Human calcium-sensing receptor (CaSR) is a G-protein-coupled receptor (GPCR) that senses small fluctuations of extracellular levels of Ca2+ ions in the blood. It maintains Ca2+ homeostasis by the modulation of parathyroid hormone (PTH) secretion from parathyroid cells and the regulation of Ca2+ reabsorption by the kidney. Like most class C GPCRs, CaSR functions as a disulphide-linked homodimer. In this study, we have determined the cryo-EM structures of CaSR in the fully inactive and agonist+PAM bound states.

To obtain the structure of the receptor in the agonist+PAM bound state, we collected a dataset of detergent solubilized full-length CaSR in the presence of PAM cinacalcet, 10 mM calcium and the compound TNCA. We have observed two active conformations with overall resolutions of 2.99 Å and 3.43 Å. The agonist+PAM bound structure of CaSR displays a substantial compaction compared to the inactive structure, including the reduction of length, height, and width. Moreover, their width changed most obviously because there are four interfaces with interaction between the two protomers at each of LB1 domain, LB2 domain, CRD, and 7TM domains, both VFT modules adopt closed–closed conformation, and the TNCA and Ca2+ ion composite is bound at the interdomain cleft between LB1 domain and LB2 domain. The cryo-EM map of active state presents a distinct density at the ligand-binding cleft of each protomer, which enabled us to unambiguously model TNCA. Two sites were previously reported, while a new Ca2+-binding site was found at the interdomain cleft of the VFT module that is close to the hinge loop and abuts the TNCA binding site, and interacts with both LB1 and LB2 domains to facilitate ECD closure. The bound Ca2+ ion is primarily coordinated with side chains of D190 and E297, carbonyl oxygen atoms of P188 backbone, and hydroxyl groups of S170 and Y489. Our CaSRagonist+PAM structure shows that TNCA and a newly identified Ca2+ ion bind at the interdomain cleft of the VFT module, and they both interact with both LB1 and LB2 domains to facilitate ECD closure, therefore forming the closed state of the ligand-binding domain required for CaSR activation. The agonist+PAM bound structure shows a TM6–TM6 interface, contacting at the apex of TM6 helices, which is a hallmark of GPCR activation (Koehl et al., 2019). In the agonist+PAM bound state, the loop of ECL2 is pulled up by the interaction among E759, W590, and K601, leading to the movement of ECL2, which would raise the reorientation of TM5 and TM6 domains during the activation of CaSR.

>YGPDQRAQKKGDIILGGLFPIHFGVAAKDQDLKSRPESVECIRYNFRGFRWLQAMIFAIEEINSSPALLPNLTLGYRIFDTCNTVSKALEATLSFVAQNKIDSLNLDEFCNCSEHIPSTIAVVGATGSGVSTAVANLLGLFYIPQVSYASSSRLLSNKNQFKSFLRTIPNDEHQATAMADIIEYFRWNWVGTIAADDDYGRPGIEKFREEAEERDICIDFSELISQYSDEEEIQHVVEVIQNSTAKVIVVFSSGPDLEPLIKEIVRRNITGKIWLASEAWASSSLIAMPQYFHVVGGTIGFALKAGQIPGFREFLKKVHPRKSVHNGFAKEFWEETFNCHLQEGAKGPLPVDTFLRGHEESGDRFSNSSTAFRPLCTGDENISSVETPYIDYTHLRISYNVYLAVYSIAHALQDIYTCLPGRGLFTNGSCADIKKVEAWQVLKHLRHLNFTNNMGEQVTFDECGDLVGNYSIINWHLSPEDGSIVFKEVGYYNVYAKKGERLFINEEKILWSGFSREVPFSNCSRDCLAGTRKGIIEGEPTCCFECVECPDGEYSDETDASACNKCPDDFWSNENHTSCIAKEIEFLSWTEPFGIALTLFAVLGIFLTAFVLGVFIKFRNTPIVKATNRELSYLLLFSLLCCFSSSLFFIGEPQDWTCRLRQPAFGISFVLCISCILVKTNRVLLVFEAKIPTSFHRKWWGLNLQFLLVFLCTFMQIVICVIWLYTAPPSSYRNQELEDEIIFITCHEGSLMALGFLIGYTCLLAAICFFFAFKSRKLPENFNEAKFITFSMLIFFIVWISFIPAYASTYGKFVSAVEVIAILAASFGLLACIFFNKIYIILFKPSRNTIEAAADYKDDDDK[2x]>[2x]TQLPPIPATHTGSGTGVAENPEENTLATAKEQGDEQEWSLILV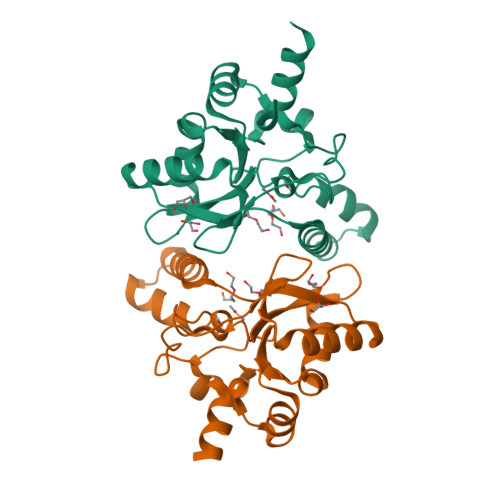NRQNPIPAQYDVELEQLSNGERIDIRISPYLQDLFDAARADGVYPIVASGYRTTEKQQEIMDEKVAEYKAKGYTSAQAKAEAETWVAVPGTSEHQLGLAVDINADGIHSTGNEVYRWLDENSYRFGFIRRYPPDKTEITGVSNEPWHYRYVGIEAATKIYHQGLCLEEYLNTEKLEHHHHHH>MRRNIFCLACLWIVQACLSLDRADILYNIRQTSRPDVIPTQRDRPVAVSVSLKFINILEVNEITNEVDVVFWQQTTWSDRTLAWNSSHSPDQVSVPISSLWVPDLAAYNAISKPEVLTPQLAHVVSDGEVQYTPSIRQRFSCDVSGVDTESGATCRIKIGSWTHHSREISVDPTTENSDDSEYFSQYSRFEIL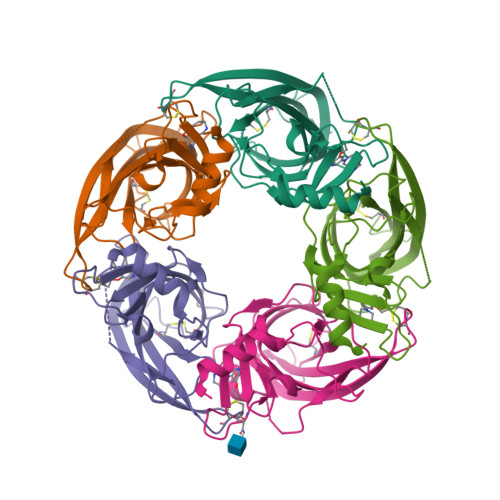DVTQKKNSVTYSCCPEAYEDVEVSLNFRKKGRSEIL[5x]MDHAR reduces the monodehydroascorbate (MDHA) radical to AsA at the expense of an NAD(P)H molecule, with NADH being the preferred donor. We report, for the first time, the crystal structure of MDHAR of O. sativa L. japonica (OsMDHAR) to understand its detailed mechanism. Structural comparison of OsMDHAR to other proteins, using the DALI server, indicated that it has the same fold as that of putidaredoxin reductase (Pdr), biphenyl dioxygenase (BphA4)18 and rubredoxin reductase (RdxR). All these proteins consist of three domains: an NAD(P)-binding domain, an FAD-binding domain, and a C-terminal domain, as shown in Figs 1 and 2.

To elucidate the detailed mechanism of the electron pathway adopted by OsMDHAR, we co-crystallized OsMDHAR with AsA, which is the final product of the enzyme, in the presence of NAD. We determined the structure of the catalytically compromised Y349F mutant in complex with AsA. Superposition of the Tyr349 and Phe349 of apo and mutant structure indicates that there is no conformational change of Phe349. However, we did not observe any large conformational changes in the structure of the OsMDHAR-NAD-AsA complex. The active site of OsMDHAR consists of highly positively charged electrostatic potential pockets, which easily bind to the negatively charged AsA, as shown in Fig. 6a. Structural studies revealed three highly conserved residues, G72, R320, and R351, positioned closed to the AsA molecule. Of these residues, Arg320 forms a hydrogen bond with AsA bound to the structure. Therefore, we suggest that R320 is important for substrate binding. The catalytic hydroxyl group of the active site Y349 residue was positioned within reasonable distance to be able to transfer electrons to O3 of AsA or ISD. The structural and mutagenesis studies suggest that the electron is transferred from the flavin N atom to the FAD flanking Tyr349, which subdivides the distance between FAD and AsA into two shorter segments of 5.7 and 3.8 Å, and then directly to the substrate, MDHA.

>[2x]HHHHHHASENLYFQGAMASEKHFKYVILGGGVAAGYAAREFAKQGVKPGELAIISKEAVAPYERPALSKGYLFPQNAARLPGFHVCVGSGGERLLPEWYSEKGIELILSTEIVKADLASKTLTSAVGATFTYEILIIATGSSVIKLSDFGTQGADSNNILYLREVDDADKLVAAIQAKKGGKAVIVGGGYIGLELSAALKINDFDVTMVFPEPWCMPRLFTADIAAFYESYYTNKGVKIVKGTVAVGFDADANGDVTAVNLKNGSVLEADIVVVGVGGRPLTTLFKGQVAEEKGGIKTDAFFETSVPGVYAVGDVATFPMKMYNELRRVEHVDHARKSAEQAVKAIKGKESGESVVEYDYLPYFFSRSFDLGWQFYGDNVGDTILFGDSDPTSAKPKFGSYWIKDGKVLGAFLEGGSPDENKAIAKVAKTQPPVANIEELKKEGLQFASKI> GSHMPKKKIQLHAEHALYDALMILNIVK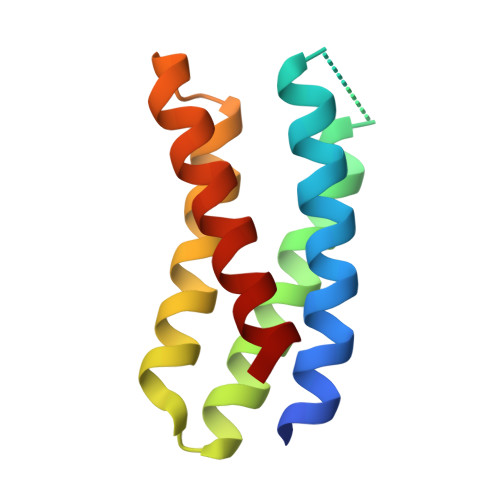TNSPPAEEKLEDYAFNFELILEEIARLFESGDQKDEAEKAKRMKEWMKRIKTTASEDEQEEMANAIITILQSWIFS>[4x]MEYRYDDNATNVKAMKYLIEHYFDNFKVDSIEIIGSGYDAVAYLVNNEYIFKTKFSTNKKKGYAKEKAIYNFLNTNLETNVKIPNIEYSYISDELSILGYKEIKGTFLTPEIYS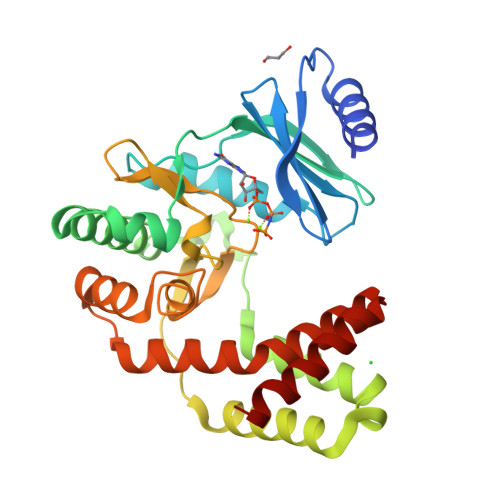TMSEEEQNLLKRDIASFLRQMHGLDYTDISECTIDNKQNVLEEYILLRETIYNDLTDIEKDYIESFMERLNATTVFEGKKCLCHNDFSCNHLLLDGNNRLTGIIDFGDSGIIDEYCDFIYLLEDSEEEIGTNFGEDILRMYGNIDIEKAKEYQDIVEEYYPIETIVYGIKNIKQEFIENGRKEIYKRTYKD>MDRSLRPEEIEELREAFREFDKDKDGYINCRDLGNCMRTMGYMPTEMELIELSQQINMNLGGHVDFDDFVELMGPKLLAETADMIGVKELRDAFREFDTNGDGEISTSELREAMRALLGHQVGHRDIEEIIRDV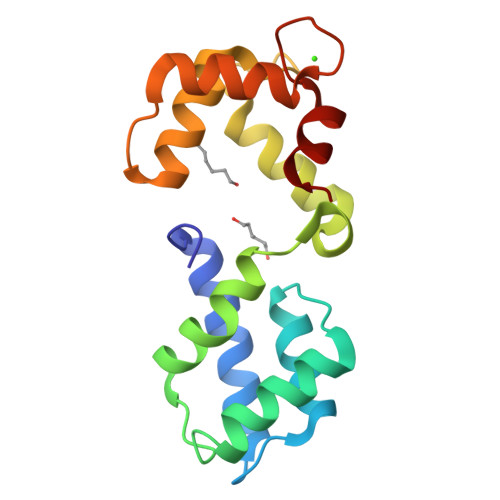DLNGDGRVDFEEFVRMMSR[6x]>NGLTYCTHASGFSFNPQTADAGTSMNVVTEQIYNKLFDIKNHSATLTPMLAQSYSISADGKEILLNLRHGVKFHQTPWFTPTRDFNAEDVVFSINRVLGHNTYLPTLAEANVTYSNPQYKVFHEQARKVRFPYFDSIKLNEKIKSVTALSPYQVKIELFAPDS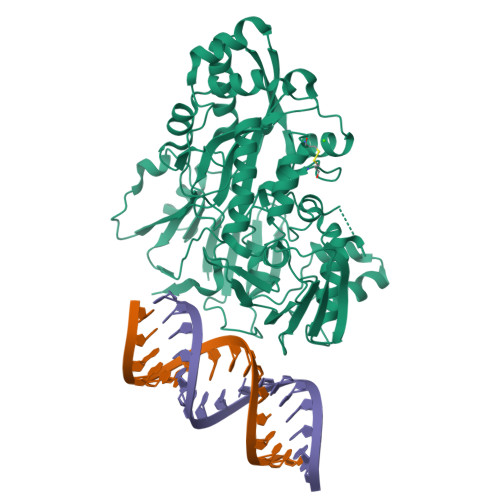SILSHLASQYAIIFSQEYAYQLSADDNLAQLDTHPVGTGPYQVKDYVYNQYVRLVRNENYWKKEAKIEHIIVDLSTDRSGRLVKFFNNECQIASYPEVSQIGLLKNDDKHYYMQSTDGMNLAYLAFNFDKPLMRDHEIRAAISQSLNRARIIHSIYHNTATVANNIIPEVSWASTVNTPEFEFDYHPKIAKNKLADKNLLLNLWVINEEQVYNPAPFKMAEMIKWDLAQAGVKVKVRAVTRPFLTAQLRNQSENYDLILSGWLAGNLDPDGFMRPILSCGTKNELTNLSNWCNEEFDQFMDRAITTSHLSSRAKAYNEAQELVLRELPIIPIANVKRILVANSRVKGVKMTPFGSLDFSTLYFI[2x]6-CHLORO-4-(CYCLOHEXYLOXY)-3-ISOPROPYLQUINOLIN-2(1H)-ONE 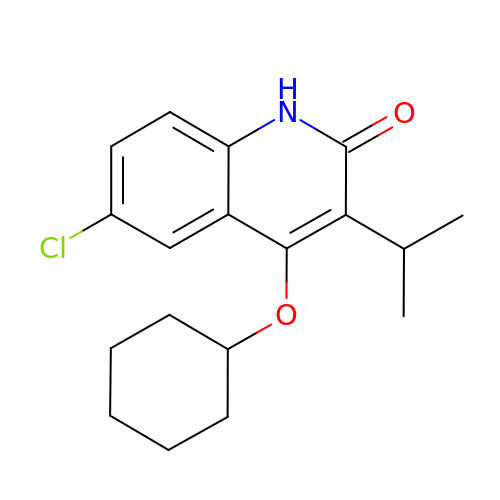| C18 H22 Cl N O2 | OQCFORGSZJSAEL-UHFFFAOYSA-N> LKESYLEESCSTITEGYLSVLRTGW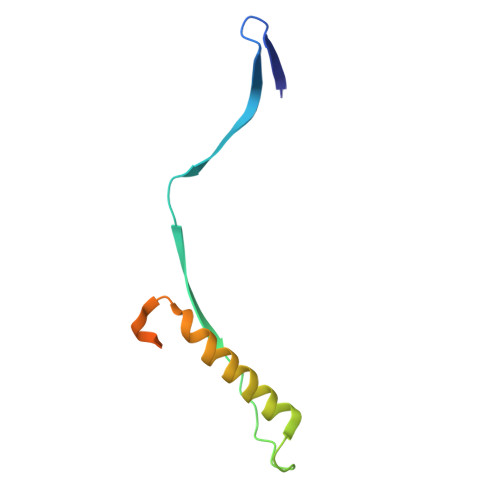YTNVFTLEVGDVENLTCADGPSLIKTELDLTKSALRELRTVSADQLAREEQIENPRQSKKRKRR>SRVVFIELKQKGVMWEGALHDARLREGADFWLSVRSSMPGHELQT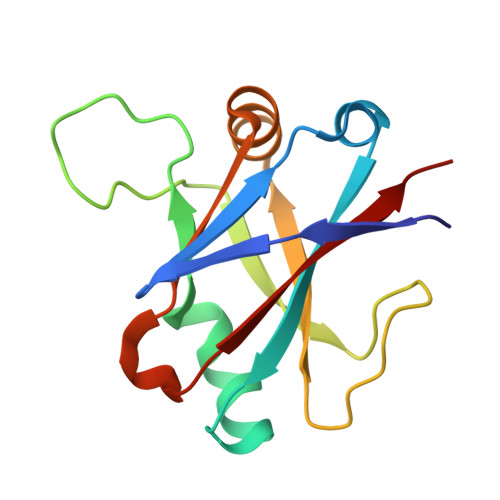KFPQLCKAGSPDDVSEVVNVALSGVIIRPVTHVPAAIPLRLENQYFALDLSTDAARAMLDAGRCTFYTPASLGDVKLELFAVLRT[2x]>[2x]KLESPGFMVHKKLKSMSQSYGVMMTGVPAEVLGQMQAERSIPSINKTGNLKQQIAKEV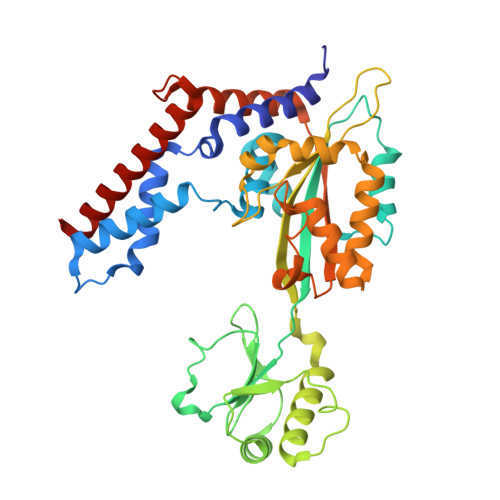SKVCHMMTEPTQSCGQASNDVCELLLGKIEAEKFHFTKYEALSADGDNLKNVLENTAPSSTNLLIRFEIDREDPPIVLVKTKNENFNPETAVKNKIYLLENKLYFIDKMGNLFNLGPGKKKCTQLFNAIGDSAEYSLCDPFVLEEPEKPEDFAISEIVDIFNEQKERFDFWIGSHSFTIYIPQTLGESPRQFYPYQAYFGSHTLQDWFVSDKDEYLSRIGIDKYIEKLAVLGKTTNTKERSDIYAEFFSKRGREAFFCAHLNEKRQPLRVKFKITEINPELALKNLQETQEFIDTHPGENPSDKVENYRNRAKLAMTEHLESLLDI>SKLNLSTEPCDVSDIECISKATQVFLDNTYQGIPEYNIKKLDPITIPSLEKSIEKINLNVRYNNLKVTGFKNQKISHFTLVRDTKAVNFKTKVNFTAEGKLVIELPKSSKTYTGEVTIEASAEGGAAYSYSVKTDDKGVEHYEAGPETVSCEIFGEPTLSVSSTLEDALKLDSDFKKIFTEYGKQLTEGRKQTACRIVETVYAVSVHNIRAA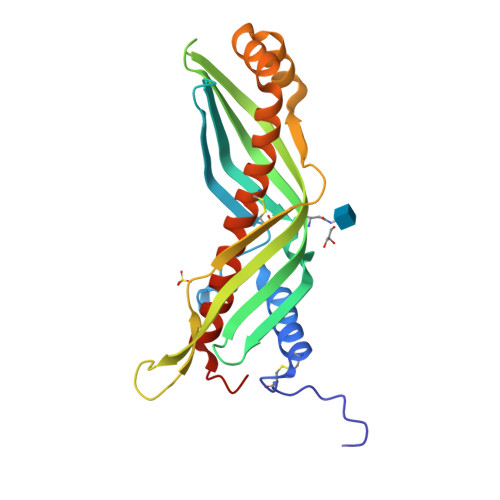ARILPKSAYFKNV[2x]>XQARSDIEKLKEAIRDTNKAVQSVQSSIGNLIVAIKSVQDYVNKEIVPSIARX[9x];>XVALDPIDISIVLNKI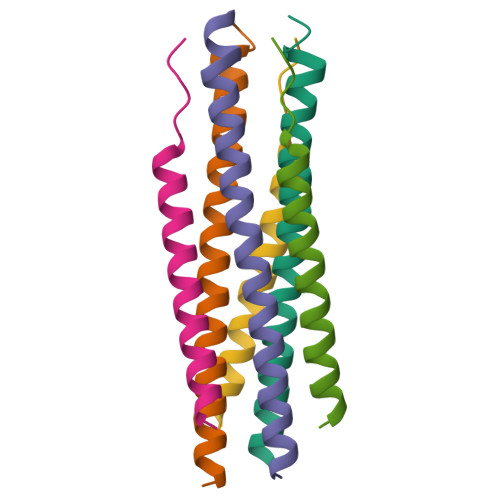KSDLEESKEWIRRSNQKLDSIX[9x]> SNAMTIAVDFDGTIVEHRYPRIGEEIPFAVETLKLLQQEKHRLILWSVREGELLDEAIEWCRARGLEFYAANKDYPEEERDHQGFSRKL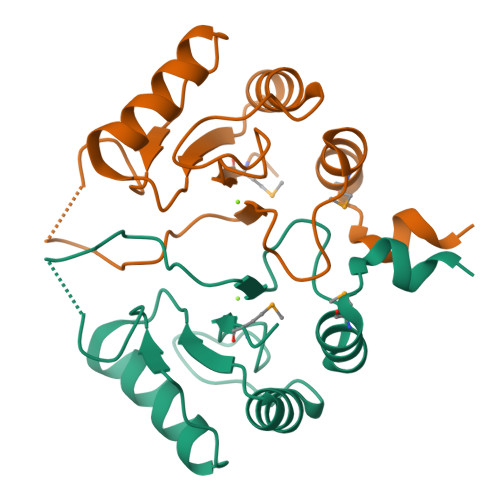KADLFIDDRNVGGIPDWGIIYEMIKEKKTFADIYSQQREENTSQKKKRKWLPF> MGRGKVKPNRKSTGDNSNVVTMIRAGSYPKVNPTPTWVRAIPFEVSVQSGIAFKVPVGSLFSANFRTDSFTSVTVMSVRA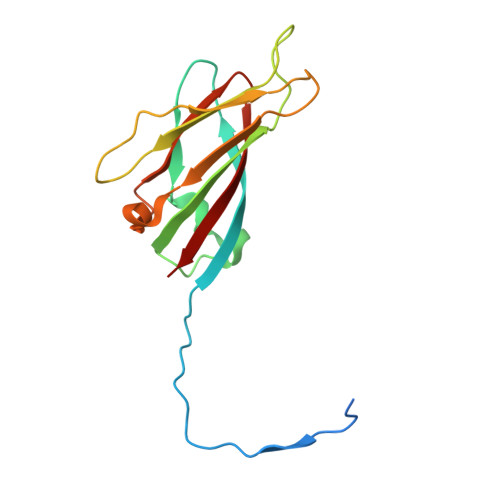WTQLTPPVNEYSFVRLKPLFKTGDSTEEFEGRASNINTRASVGYRIPSNLRQNTVAADNVCEVRSNCRQVALVISCCFN>[2x]MVAPLLK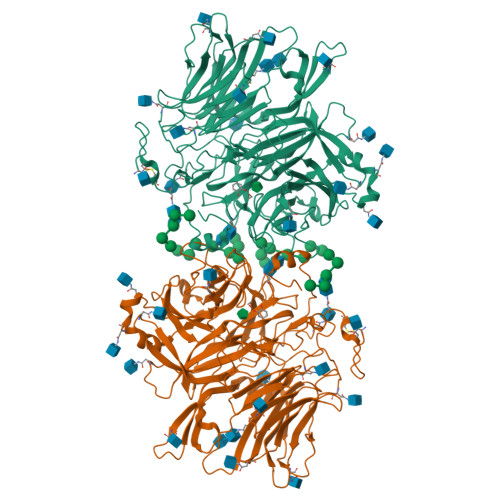TLPFLAAAYAAELDLPNFSALNRRQDNSTSSSAGCSLDQTVAPGNLTLCGNATLFTTFRPKARFIAPEGWMNAPMGLYQRADGSIHAGYQSHPKHIQWGNISQGAAYSSDFTSWTDFNGSEGYKTIWPSQIYDIRGVFDGSIIKEGIDGYPTILYTSTSFGPLGATLNEAEGTETQSLAYTTDDGASWIKLGYGAGQNPVIYEWPETNLTGFRDPYVFQSPRLEALLANTTSITNATGDHFATISGGVHGDGARLFLYRQHTTGEFIKWTYLGPLVTTGYKESYGEWSGNYGINFETAGVTRLNPAGAAWDNGSDTTAVDFVTFGTEQGRADHQNHWPLWAAVDYEVRDNGSIEAVIAYSGVQDWGRSYAYASFPVEGYRQVSVGWIYEDDDNVILAKQFGYQGAFTLFRDLFVKVVENVSPSTPGLFEQASWSTKNSTDGMSVTVTTLGQRVVPETLAAYKGNSTVSTLAPVMLNESAAAYTPFSSQPTDRFYALTGSFEFGLNTTAKAGFRVLASEEEYTDIWFDPASENLTVVRTASSLIKSFGNDTELAKVKLYEIVGAESKTLNLTVFVDGSVIEIYANDEVALSTRAYPWLANSTGAGLLADGTTAGDVVGVSGLELWDGLVDAWPARPANTSQGLVWDGPTAAMYGLFAGY>[2x]MDEARKLKIAAAAEALTHV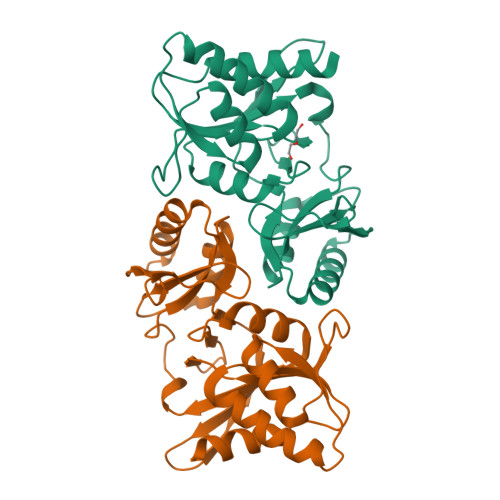KDGMRLGIGTGSTAEEFVRLLADKVSNGFKIIGVPTSERTAKLCKELGVPLTTLDETPHLDLTVDGADEVDTNLSLIKGGGGALLREKIVAAASDAMIVIADSSKVVETLGRFPLPVEVNRFGLGATMRAIEEAAAKCGLAGPLALRLKDGSPFVTDGGHYIVDASFGRIPDPKTLSDALFAIPGVVEHGLFIGLARAAVVAGNDGIRTMNRS>MRGSHHHHHHGIDHMPVEGSEEDKSQTGVNRASKGGLIYGNYLHLEKVLNAQELQSETKGNKIHDEHLFIITHQAYELWFKQILWELDSVREIFQNGHVRDERNMLKVVSRMHRVSVILKLLVQQFSILETMTALDFNDFREYLSPASGFQSLQFRLLENKIGVLQNMRVPYNRRHYRDNFKGEENELLLKSEQEKTLLELVEAWLERTPGLEPHGFNFWGKLEKNITRGLEEEFIRIQAKEESEEKEEQVAEFQKQKEVLLSLFDEKRHEHLLSKGERRLSYRALQGALMIYFYREEPRFQVPFQLLTSLMDIDSLMTKWRYNHVCMVHRMLGSKAGTGGSSGYHYLRSTVSDRYKVFVDLFNLSTYLIPRHWIPKMNPTIHKFLYTAEYCDSSYFSSDESD[4x]

Tryptophan-2,3-dioxygenase (TDO2) and indoleamine-2,3-dioxygenase (IDO1) are structurally distinct heme enzymes that catalyze the conversion of L-tryptophan to N-formyl-kynurenine, and play important roles in metabolism, inflammation, and tumor immune surveillance. Tryptophan-2,3-dioxygenase (TDO2) and indoleamine-2,3-dioxygenase 1 (IDO1) catalyze the same reaction: the conversion of L-tryptophan (Trp) to N-formyl-kynurenine (NFK). Both enzymes evolved to bind heme for substrate binding and catalysis but are structurally distinct: IDO1 is monomeric, while TDO2 is tetrameric with two independent TDO2 molecules contributing to each of its four active sites. The enzymes can adopt an inactive, heme-free (apo) state or an active, heme-containing (holo) state, with the balance between them varying dynamically according to biological conditions. While apo-TDO2 is catalytically inactive, the term “apo-TDO2 inhibitor” is used to describe compounds that bind to apo-TDO2, compete with heme binding and thus prevent the formation of enzymatically active holo-TDO2.

The 2.61 Å resolution structure of Cpd-2 in complex with apo-TDO2 revealed the inhibitor bound to the active site (including the heme binding pocket) of all four TDO2 molecules of the homo-tetramer. Cpd-2 is a mixture of two diastereomers, of which only ethyl (R)-9-(3-(2-isopropylphenyl)-1-((S)-1-phenylethyl)ureido)-2-methoxy-4-oxo-6,7,8,9-tetrahydro-4H-pyrido[1,2-a]pyrimidine-3-carboxylate was observed in the co-crystal structure. Cpd-2 occupies both the heme and substrate binding pockets of the active site and, in keeping with its potent inhibition of TDO2 activity in the cellular assay, forms multiple binding interactions with TDO2. Both benzyl rings of the inhibitor are bound in hydrophobic pockets formed by phenylalanine, leucine and tryptophan side chains. The benzyl rings are bridged by a central urea linker that forms hydrogen bonds with the side chains of His328 and His76 (both are key residues for holo-TDO2 activity, with His328 anchoring the heme via its iron atom and His76 binding the substrate Trp). The backbone nitrogen of Ser155 forms an additional bifurcated hydrogen bond interaction with the inhibitor. The larger fused ring substituent of the inhibitor binds between loop 145–155 and His328 and may serve to stabilize the loop conformation and shield the hydrogen bond between the inhibitor and His328 from competing water molecules. Residues Phe72, His76 and His328 are shifted away from the inhibitor by 1.0-1.5 Å, together with the neighboring residues of the associated alpha-helices. The shortest distance between the His76 and His328 side chain atoms is 4.0 Å in apo-TDO2 and 6.9 Å in the Cpd-2 / apo-TDO2 complex. AMT was also observed in the structure of Cpd-2 bound to apo-TDO2, with an identical binding mode.> HHHSSGLEVLFQGPGSEFATTLPDGAAAESLVESSEVAVIGFFKDVESDSAKQFLQAAEAIDDIPFGITSNSDVFSKYQLDKDGVVLFKKFDEGRNNFEGEVTKENLLDFIKHNQLPLVIEFTEQTAPKIFGGEIKTHILLFLPKSVSDYDGKLSNFKTAAESFKGKILFIFIDSDHTDNQRILEFFGLK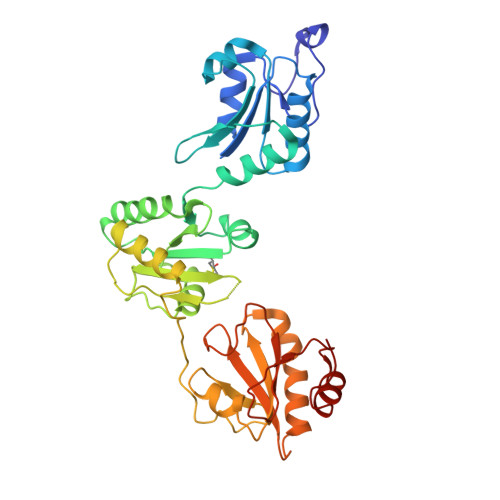KEECPAVRLITLEEEMTKYKPESEELTAERITEFCHRFLEGKIKPHLMSQELPEDWDKQPVKVLVGKNFEDVAFDEKKNVFVEFYAPWCGHCKQLAPIWDKLGETYKDHENIVIAKMDSTANEVEAVKVHSFPTLKFFPASADRTVIDYNGERTLDGFKKFLESGGQDGAG> MASSGTTSTRKR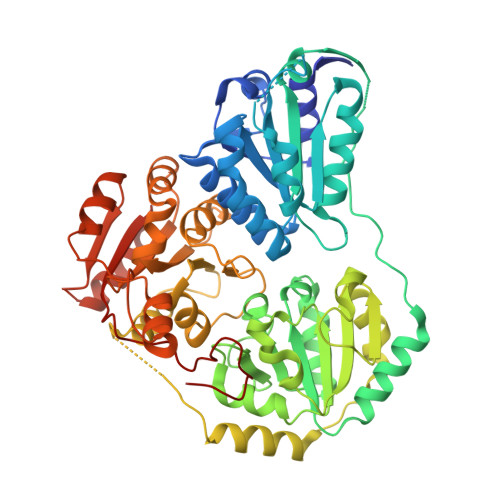FTGAEFIVHFLEQQGIKIVTGIPGGSILPVYDALSQSTQIRHILARHEQGAGFIAQGMARTDGKPAVCMACSGPGATNLVTAIADARLDSIPLICITGQVPASMIGTDAFQEVDTYGISIPITKHNYLVRHIEELPQVMSDAFRIAQSGRPGPVWIDIPKDVQTAVFEIETQPAMAEKAAAPAFSEESIRDAAAMINAAKRPVLYLGGGVINAPARVRELAEKAQLPTTMTLMALGMLPKAHPLSLGMLGMHGVRSTNYILQEADLLIVLGARFDDRAIGKTEQFCPNAKIIHVDIDRAELGKIKQPHVAIQADVDDVLAQLIPLVEAQPRAEWHQLVADLQREFPCPIPKACDPLSHYGLINAVAACVDDNAIITTDVGQHQMWTAQAYPLNRPRQWLTSGGLGTMGFGLPAAIGAALANPDRKVLCFSGDGSLMMNIQEMATASENQLDVKIILMNNEALGLVHQQQSLFYEQGVFAATYPGKINFMQIAAGFGLETCDLNNEADPQASLQEIINRPGPALIHVRIDAEEKVYPMVPPGAANTEMVGE Long-term immune evasion by the African trypanosome is achieved through repetitive cycles of surface protein replacement with antigenically distinct versions of the dense Variant Surface Glycoprotein (VSG) coat. The mature VSG proteins are attached to the cell surface by a GPI-anchor, and consist of two main regions: (1) a large, N-terminal domain (NTD) of roughly 300–400 amino acids that is most distal to the membrane and (2) a smaller, membrane-proximal C-terminal domain (CTD) spanning 80–120 amino acids beneath the NTD that harbors the GPI-anchor. Therefore, at the heart of antigenic variation in the African trypanosome are the NTDs of the VSGs. These large subdomains are elongated folds centered on a three-helix bundle scaffold.

The third crystal form (VSG11WT-AS grown in ammonium sulfate and solved to 1.75Å resolution) contains two molecules in the asymmetric unit. However, these two monomers are not arranged in a standard class A type dimeric arrangement in which the three-helix bundles, top, and bottom lobes align alongside each other, but are instead “tail-to-tail” with the lower lobe of one monomer interacting with the lower lobe of the other. In contrast, the crystal packing is characterized by a three-fold trimer identical to those seen in all the class B protein structures solved to date, including the alternative crystal forms of VSG11. Therefore, the assembly of VSG11WT-AS is most accurately described as trimeric and not dimeric (and certainly not dimers in the sense of those seen in class A VSGs), providing an interesting example in which the contents of the asymmetric unit of the crystal do not present the likely biological assembly, whereas the crystallographic arrangement does. Intriguingly, these two independent monomers are characterized by a significant conformational change in bottom lobe of the protein. This change consists of a 12-degree rotation of the bottom lobe from one monomer to the other.

>[2x]NIGTGDNVLHRAALCGIIELAGKRAKLETALPNFQNELNSILELNMTAAEPTWLDQFRDKDDRSKPRDLTKQPLPKDTNWADHWTAWAKAALPLLNDETHQAKLKEYKLAGLQPEKLERARNTIRRLTAEAVAKAQDPTVAESTADLTTEEDLQKQINQAVYSKDTEPDDDFNGYTAFEGKASTNRQTICGSAVAGSKATNAMDALFCVCADDRTNGADAGKACVAGTAPGTGWNPGVTATPTGTMLQKVRKLCNTHGKTTLSAAAIEGRLTAVGNLLTRGSATSILGSFLATDCSGDQGSGMCVAYTEVTDAKGTPTKDIPWMQKLDSVRIKLQKHERAVEKLGKPQHDLKTILTLAKDPAYLQLASVGTRHLETTKQRVSNEQGKTQQTQQTCEQYNNKKNDCVKTGVCKWEE> MAAQQCNGIYIWKIGNFGMHLKCQEEEKPVVIHSPGFYTGKPGYKLC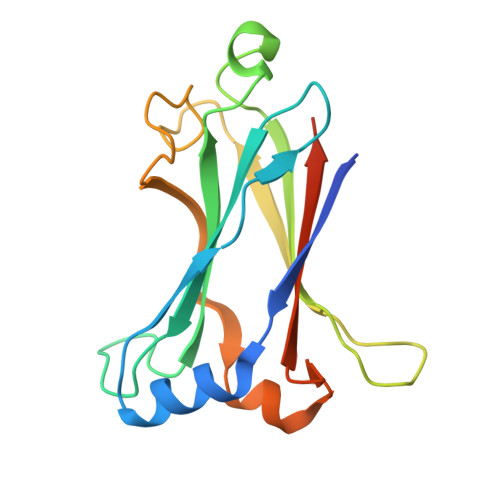MRLHLQLPTAQRCANYISLFVHTMQGEYDSHLPWPFQGTIRLTILDQSEAPVRQNHEEIMDAKPELLAFQRPTIPRNPKGFGYVTFMHLEALRQRTFIKDDTLLVRCEVSTRFDLEHHHHHH>GAMAHSDTVEFYQRLSTETLFFIFYYLEGTKAQYLAAKALKKQSWRFHTKYMMWFQRHEEPKTITDEFEQGTYIYFDYEKWGQRKKEGFTFE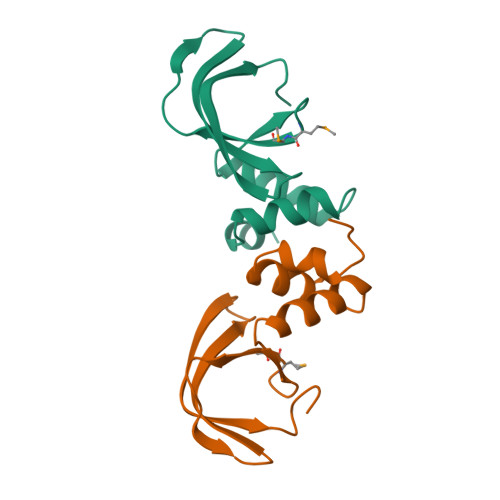YRYLEDRDLQ[6x]> XELL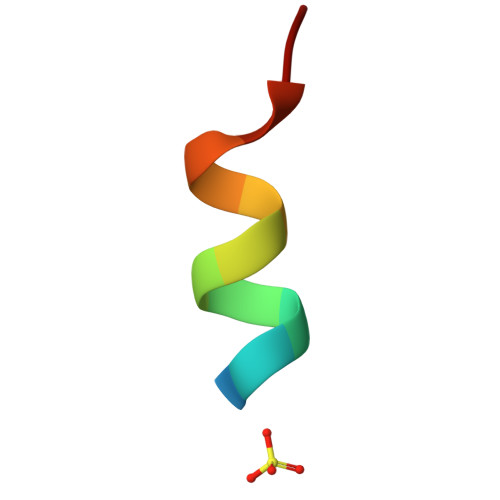KKLLEELKG> GAMGSKQFDYIIIGGGSAGAVVANRLSEDSGTSVLLLEAGGSDMHPFTRIPAGSALAIASPKFNWMYDVEPDPSRDGRVDIWPAGKVLGGGSSINGMMFVRGNAWDYDLWAQKGATGWDYAGVLPYFRKMESYALGSDDWRGGQGPQHVDRTRVPNELTDLWVKSAEKIGIRRNDDLN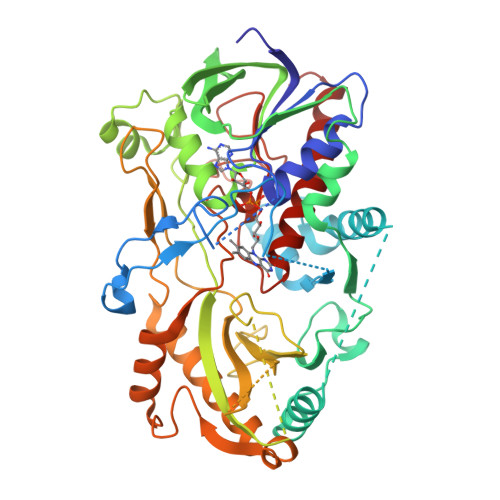GASQEGVGYCDASQKDGWRHSTAQAYIRGIKGKRANFTLELKAFVERIIIEGGRAVGVRYSKNGRGMEVRARKGVVLSAGAIASPKLLLLSGIGPAEELAQHEIPMVVDSPDVGANLQEHPAVIMSFHVNKPSLGANRNPVSDLLHGMNFIFRGRGPLTTGIGHAQALVKTDDRYAAPNVQLIISPFSYDFDERGPKLYNKPSVGLAVGLARPESRGTVRLKSADPKDKPLINYPLLGEQSEVDQMVAGCRILRKIAHAEPFRDVLVDERLPGAEVESDAELERYIRQFAFPMYHVSCSCRMGSDPASVVDPELRVRGVSGLWVVDASVMPTLPAGNINASAIMIGERGADLIKQQAKTPETVQ>MPERLQVYKCEVCGNIVEVLNGGIGELVCCNQDM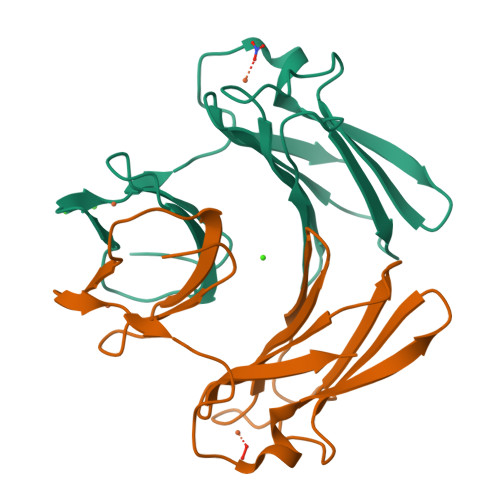KLMSENTVDAAKEKHVPVIEKIDGGYKVKVGAVAHPMEEKHYIQWIELLADDKCYTQFLKPGQAPEAVFLIEAAKVVARAYCNIHGHWKAEN[4x]>[2x]MSEGRRGLGRGLSALLGEVDAAPAQAPGEQLGGSREAPIEILQRNPDQPRRTFREEDLEDLSNSIREKGVLQPILVRPSPDTAGEYQIVAGERRWRAAQRAGLKTVPIMV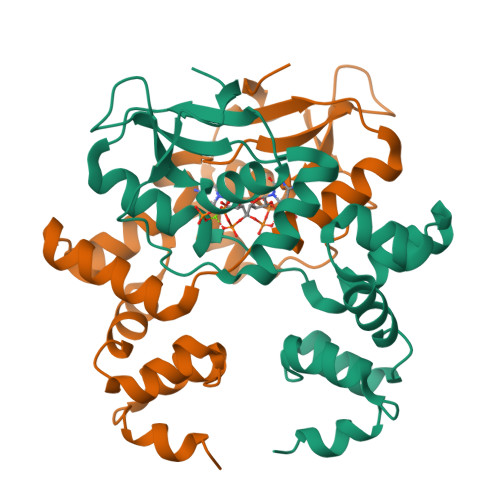RELDDLAVLEIGIIENVQRADLNVLEEALSYKVLMEKFERTQENIAQTIGKSRSHVANTMRLLALPDEVQSYLVSGELTAGHARAIAAAADPVALAKQIIEGGLSVRETEALARKAPNLSAGKSKGGRPPRVKDKLAAALEHHHHHH> DISTLPRVKVDLVKPPFVHAHDQVAKTGPRVVEFTMTIEEKKLVIDREGTEIHAMTFNGSVPGPLMVVHENDYVELRLINPDTNTLLHNIDFHAATGALGGGALTQVNPGEETTLRFKATKPGVFVYHCAPEGMVPWHVTSGMNGAIMVLPRDGLKDEKGQPLTYDKIYYVGEQDFYVPKDEAGNYKKYETPGEAYEDAVKAMRTLTPTHIVFNGAVGALTGDHALTAAVGERVLVVHSQANRDTRPHLIGGHGDYVWATGKFRNPPD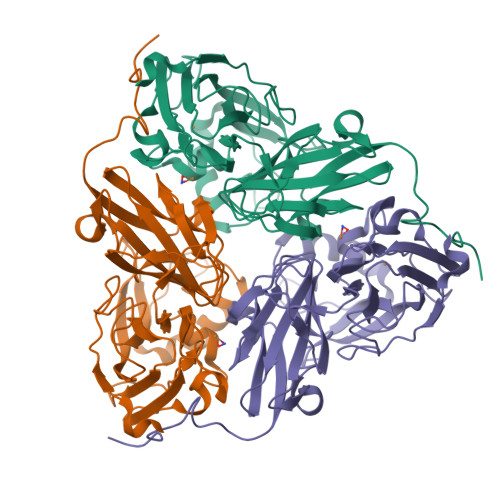LDQETWLIPGGTAGAAFYTFRQPGVYAYVNHNLIEAFELGAAGHFKVTGEWNDDLMTSVVKPASM3-[3,5-bis(fluoranyl)-4-(3-methoxyphenyl)phenyl]benzo[f]benzotriazole-4,9-dione 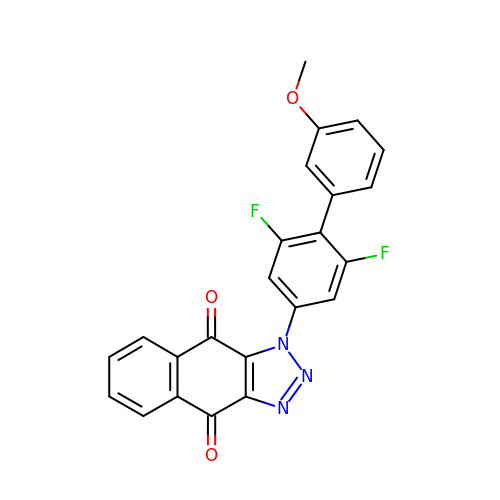| C23 H13 F2 N3 O3 | MBRGIUONQXHXCP-UHFFFAOYSA-N>MKMLYDLAKKRKTVRRFKKEKPPLEDLIYSLKVANEAPSGMNAQPWRFLIVEDEKLKGQIRRVCERSEKTFYENVRGRLKEWLDEKRFTWRKPFLKEAPYLLLVFSEKSAPYSRESVWLAVGYLLLALEEKGLGSVPYTPPDFREV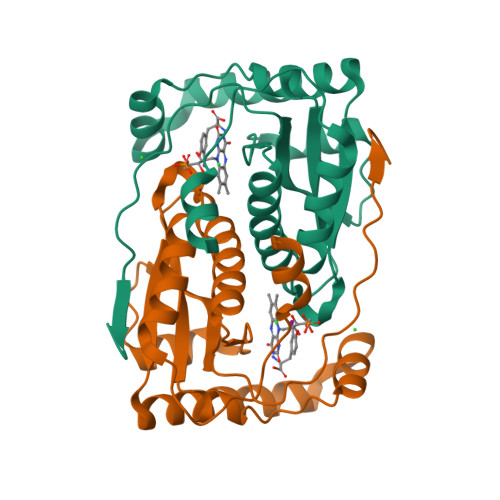EKLVNTPSELRLEVILPVGYPDDPKPKYPRNEVIVRYNTFHHHHHH[2x]> MGAVMGTFSSLQTKQRRPSKDKIEDELEMTMVCHRPEGLEQLEAQTNFTKRELQVLYRGFKNECPSGVVNEETFKQIYAQFF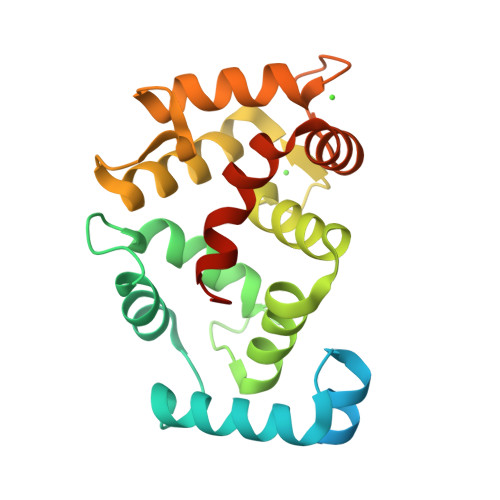PHGDASTYAHYLFNAFDTTQTGSVKFEDFVTALSILLRGTVHEKLRWTFNLYDINKDGYINKEEMMDIVKAIYDMMGKYTYPVLKEDTPRQHVDVFFQKMDKNKDGIVTLDEFLESCQEDDNIMRSLQLFQNVMVEHHHHHH>[2x]GMTDAPADAPLDADAR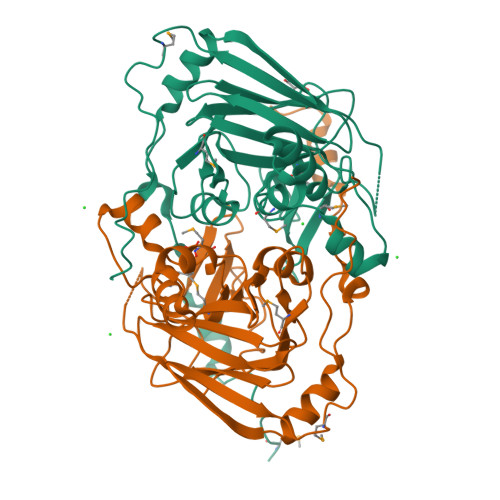RAVKPVICYPNDSLPRPDLALYRAARASARKTGEVLVPPREGRCFEVKAGQFFRISSVEGPQVGDLNLHNLHDLTERFFSGKTRALHGTHVTTGERLWSNLPYLRPMATIIEDTLGWYGIDQYGGSVHDVIGTRCDPYTGNLLAGGHYHHCCHSNLTRALADHTGLPLHEAEMLVHDVLNVFMCTGFTRDTGQYFMKASPVRPGDYLEFFAEIDLLGNLSACPGGDCSSEHSSDTASCHPLLVEIFAPAEGMLGDWPSPSVNGYDRSHGR>[2x]GAMGTKDLPIHACSYCGIHDPACVVYCNTSKK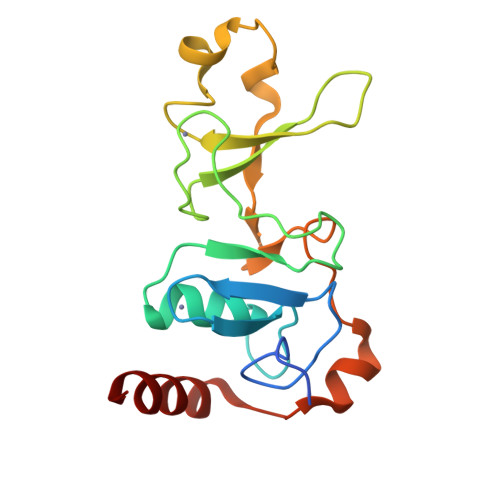WFCNGRGNTSGSHIVNHLVRAKCKEVTLHKDGPLGETVLECYNCGCRNVFLLGFIPAKADSVVVLLCRQPCASQSSLKDINWDSSQWQPLIQDRCFLSWLVKIPSEQEQLRARQITAQQINKLEELWKEN> MADVAGTSNRDFRGREQRLFNSEQYNYNSSLNGEVSVWVYAYYSDGSVLVINKNSQYKVGISETFKVLKEGSGAKPRAIQIIFSPSVNVRTIKMAKGNAVSVPDEYLQRSHPWEATGIKYRKIKRDGEIVGYSHYFELPHEYNSISLAVSGVHKNPSSYNVGSAHNVMDVFQSCDLALRFCNRYWAELELVNHYISP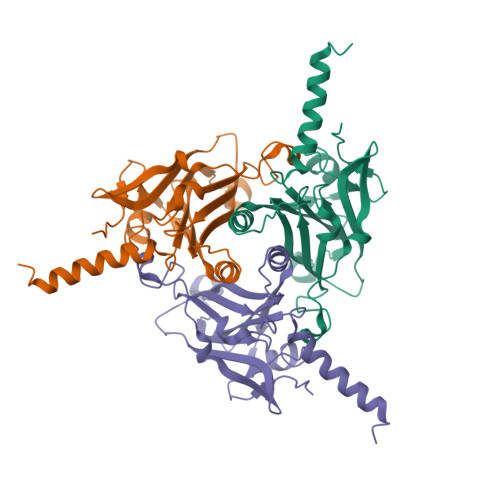NAYPYLDINNHSYGVALSNRQ ondansetron | C18 H19 N3 O | 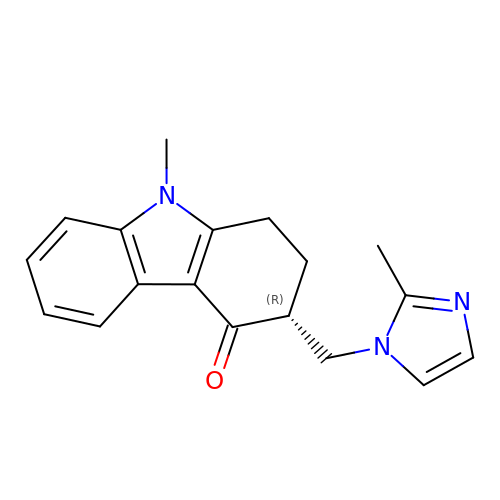FELGMEQIXOGIFQ-UHFFFAOYSA-N>[3x]RSHHHHHHGLIQERRSHEVNPAAHLTGANSSLTGSGGPLLWETQLGLAFLRGLSYHDGALVVTKAGY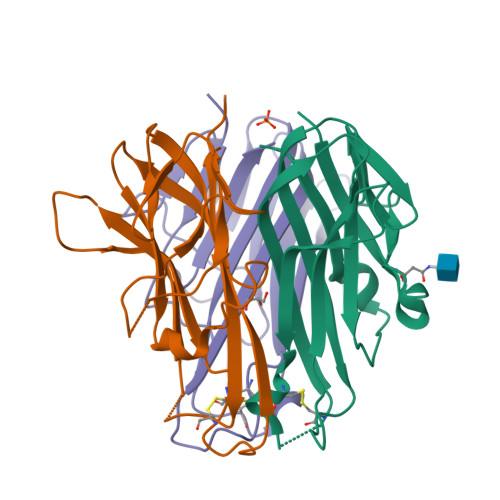YYIYSKVQLGGVGCPLGLASTITHGLYKRTPRYPEELELLVSQQSPCGRATSSSRVWWDSSFLGGVVHLEAGEEVVVRVLDERLVRLRDGTRSYFGAFMV>TSTDWKEAKSFLKGLSDKQREEHYFCKDFVRLKKIPTWKEMAKGVAVKVEEPRYKKDKQLNEKISLLRSDITKLEVDAIVNAANSSLLGGGGVDGCIHRAAGPLLTDECRTLQSCKTGKAKITGGYRLPAKYVIHTVGPIAYGEPSASQAAELR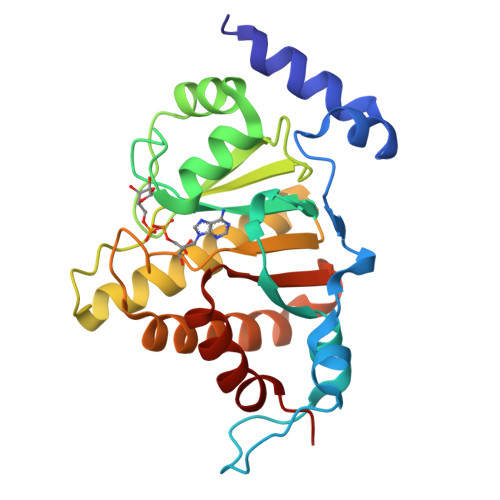SCYLSSLDLLLEHRLRSVAFPCISTGVFGYPCEAAAEIVLATLREWLEQHKDKVDRLIICVFLEKDEDIYRSRLPHYFPVA[4x]> MDSKQQCVKLNDGHFMPVLGFGTYAPPEVPRSKALEVTKLAIEAGFRHIDSAHLYNNEEQVGLAIRSKIADGSVKREDIFYTSKLWS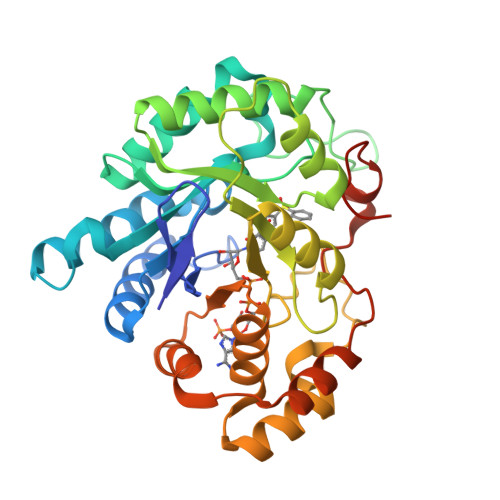TFHRPELVRPALENSLKKAQLDYVDLYLIHSPMSLKPGEELSPTDENGKVIFDIVDLCTTWEAMEKCKDAGLAKSIGVSNFNRRQLEMILNKPGLKYKPVCNQVECHPYFNRSKLLDFCKSKDIVLVAYSALGSQRDKRWVDPNSPVLLEDPVLCALAKKHKRTPALIALRYQLQRGVVVLAKSYNEQRIRQNVQVFEFQLTAEDMKAIDGLDRNLHYFNSDSFASHPNYPYSDEYLEHHHHHH>SNVPHKSSLPEGIRPSTVLRIRGLVPPNASRFHVNLLCGEEQGSDAALHFNPRLDTSEVVFNSKEQGSWGREERGPGVPFQRGQPFEVLIIASDDGFKAVVGDAQYHHFRHRLPLARVRLVEVGGDVQLDSVRIF[2x]

pmcHuman galectins (GAL) are oligomeric β-galactosidase-binding lectins assembled from small (∼15 kDa) protomeric carbohydrate recognition domains (CRD). Among prototype galectins, galectin-7 (GAL-7) is recognized for its preferential expression profiles in normal epithelial cells. For example, while extracellular GAL-7 can trigger apoptosis of activated T cells following binding to glycoreceptors via its GBS, it can also bind E-cadherin on epithelial cells independently of its GBS. In this work, we studied the impact of homodimer interface mutations on the induction of Jurkat T cell apoptosis, allowing us to positively and negatively modulate the biological activity of GAL-7 by designing a covalent disulfide bridge (G16C) and destabilizing mutation (G16S) to control homodimer strength, stability, and biological activity.

We finally prioritized individual substitutions G16S and F135S, as they caused the largest ΔΔGB among all remaining variants. Based on our computational predictions, mutations G16S and F135S should weaken GAL-7 homodimer interactions, while formation of a disulfide bridge in G16C could strengthen protomer interactions and favor GAL-7 homodimer stability. We found that both G16C and G16S variants maintain GAL-7 dimer architecture in solution, unlike other protomer interface mutations that likely perturb the hydrophobic core of the dimer interface, resulting in insoluble constructs (e.g., F135S). In contrast, the G16S variant displays 32-fold lower dimer affinity relative to WT GAL-7 (KD = 1.88 μM), indicative of significant homodimer destabilization induced by the mutation. Consistent with our MST results, G16S was found to be the least stable homodimer, with a dimer interaction energy of -11.6 ± 0.1 kcal/mol. Conversely, the G16S mutation weakens GAL-7 stability, inducing a 9.1 °C decrease in melting temperature. Our results show that the G16S mutation decreases the proapoptotic activity of GAL-7, yielding an EC50 of 13.7 μM (95% confidence interval [CI95%] between 10.2 and 18.3 μM) relative to 8.4 μM (CI95% 7.6–9.1 μM) for WT GAL-7. One of the most significant structural rearrangements between WT and G16X apo structures occurs in the local environment of residues 8–17 (loop 1), which exhibit significant atomic-scale deviations in the variants. This local rearrangement of loop 1 involves Gly16 and its neighboring residues, particularly residues Pro10, Glu11, Gly12, and Arg14.>[3x]SNAMADIRVTHEAQVTVISFPAVFQRLRETEVEQIASTFLAAMQGA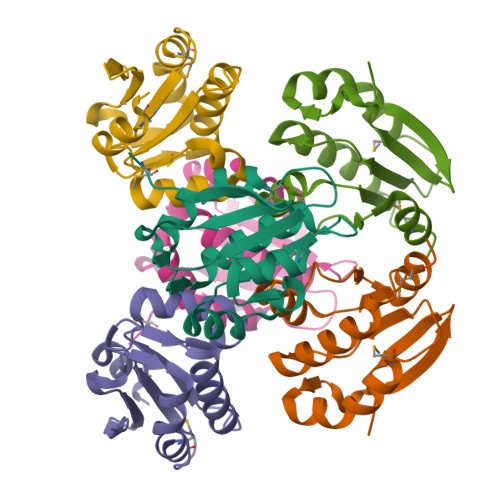QPRKVLIDLEGVEFFGSSFIELLVRGWKRIKEDQQGVFALCSVSPYCVEVLQVTHIDEVWPRYSTKQEALLAMAS>SGQNYPEEADGTLDCISMALTCTFNRWGTLLAVGCNDGRIVIWDFLTRGIAKIISAHIHPVCSLCWSRDGHKLVSASTDNIVSQWDVLSGDCDQRFRFPSPILKVQYHPRDQNKVLVCPMKSAPVMLTLSDSKHVVLPVDDDSDLNVVASFDRRGEYIYTGNAKGKILVLKTDSQDLVASFRVTTGTSNTTAIKSIEFARKGSCFLINTADRIIRVYDGREILTCGRDGEPEPMQKLQDLVNRTPWKKCCFSGDGEYIVAGSARQHALYIWEKSIGNLVKILHGTRGELLLDVAWHPVRPIIASISSGVVSIWAQNQ[2x];>DEELEDSKALLYLPIAPEVEDPEENPYGPPPDGSQPPKKKPKTTNIELQGVPNDEVHPLLGVKGDGKSK[2x]

The methyltransferase activity of MLL1 is regulated by three conserved core subunits, WDR5, RBBP5 and ASH2L. Among KMT2-associated regulators, RBBP5 and its yeast ortholog Swd1 play a pivotal role in the assembly and activity regulation of KMT2-family complexes. Both RBBP5 and Swd1 contain a WD40 propeller domain followed by a long C-terminal tail. The C-terminal tail can be further divided into two regions, a WD40 repeat proximal (WDRP) region and a C-terminal distal (CTD) region.

Selenomethionine-substituted crystals diffracted up to 1.8 Å resolution, and we were able to solve the complex structure by single-wavelength anomalous dispersion. The electron density map unambiguously allowed us to build the atomic model of the majority of RBBP5WD40 (residues 12–324) and two segments of RBBP5CTDM (residues 396–404 and 452–474). RBBP5WD40 forms a canonical β-propeller fold with seven WD40 repeats. The RBBP5WD40 conformation is almost identical to that of apo-RBBP5WD40 with a root-main-square deviation value of 0.39 Å for 319 Cα pairs, indicating that CTDM binding induces no dramatic structural rearrangement of RBBP5WD40. RBBP5CTDM exhibits an extended conformation and wraps the WD40 propeller through two segments, burying 1472 Å2 of the surface area at the interface. The first segment of RBBP5CTDM (CTD1) contains residues 396–404 and sits on the top surface of RBBP5WD40. Three leucine residues (L399, L400 and L402) in CTD1 fit snugly into the hydrophobic groove formed by residues from RBBP5WD40, including W35, L38, I50, W74, V95, L96, and the aliphatic side chain of K60. The second segment (CTD2) meanders its way around the side face of RBBP5WD40 and also pairs with the repeat 2 of the WD40 propeller to form a five-stranded β-sheet. The interface between RBBP5CTD2 and RBBP5WD40 consists of a set of hydrophobic residues, including I457, L459, V462, P469, L470 and L471 from RBBP5CTD2 and L28, C70, F106, I110, L111, P127, V133, V144 and L299 from RBBP5WD40. Combined mutation of CTD1 and CTD2 (L399A/L400A/I457A/L459A, named as RBBP5CTDM-4A mutant) further disrupted the RBBP5CTDM–RBBP52–333 interaction and reduced the HKMT activity of the MLL1 complex to the activity level comparable with that of the complete-CTD-deletion construct (RBBP52–381).> AAKRRPKEAEPEQVAPETPEDR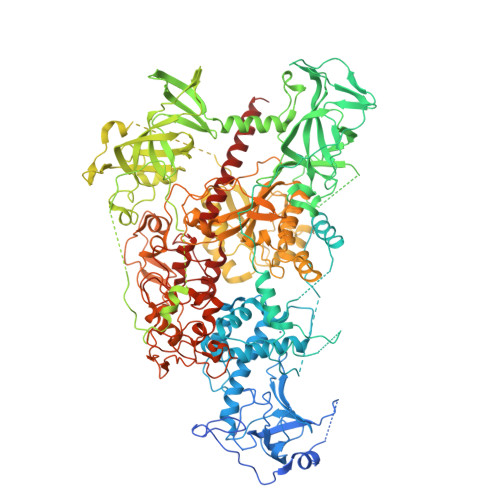DEDEREEKRRKTTRKKLESHTVPVQSRSERKAAQSKSVIPKINSPKCPECGQHLDDPNLKYQQHPEDAVDEPQMLTSEKLSIYDSTSTWFDTYEDSPMHRFTSFSVYCSRGHLCPVDTGLIEKNVELYFSGCAKAIHDENPSMEGGINGKNLGPINQWWLSGFDGGEKVLIGFSTAFAEYILMEPSKEYEPIFGLMQEKIYISKIVVEFLQNNPDAVYEDLINKIETTVPPSTINVNRFTEDSLLRHAQFVVSQVESYDEAKDDDETPIFLSPCMRALIHLAGVSLGQRRATRRVMGATKEKDKAPTKATTTKLVYQIFDTFFSEQIEKYDKEDKENAMKRRRCGVCEVCQQPECGKCKACKDMVKFGGTGRSKQACLKRRCPNLAVKEADDDEEADDDVSEMPSPKKLHQGKKKKQNKDRISWLGQPMKIEENRTYYQKVSIDEEMLEVGDCVSVIPDDSSKPLYLARVTALWEDKNGQMMFHAHWFCAGTDTVLGATSDPLELFLVGECENMQLSYIHSKVKVIYKAPSENWAMEGGTDPETTLPGAEDGKTYFFQLWYNQEYARFESPPKTQPTEDNKHKFCLSCIRLAELRQKEMPKVLEQIEEVDGRVYCSSITKNGVVYRLGDSVYLPPEAFTFNIKVASPVKRPKKDPVNETLYPEHYRKYSDYIKGSNLDAPEPYRIGRIKEIHCGKKKGKVNEADIKLRLYKFYRPENTHRSYNGSYHTDINMLYWSDEEAVVNFSDVQGRCTVEYGEDLLESIQDYSQGGPDRFYFLEAYNSKTKNFEDPPNHARSPGNKGKGKGKGKGKGKHQVSEPKEPEAAIKLPKLRTLDVFSGCGGLSEGFHQAGISETLWAIEMWDPAAQAFRLNNPGTTVFTEDCNVLLKLVMAGEVTNSLGQRLPQKGDVEMLCGGPPCQGFSGMNRFNSRTYSKFKNSLVVSFLSYCDYYRPRFFLLENVRNFVSYRRSMVLKLTLRCLVRMGYQCTFGVLQAGQYGVAQTRRRAIILAAAPGEKLPLFPEPLHVFAPRACQLSVVVDDKKFVSNITRLSSGPFRTITVRDTMSDLPEIQNGASNSEIPYNGEPLSWFQRQLRGSHYQPILRDHICKDMSPLVAARMRHIPLFPGSDWRDLPNIQVRLGDGVIAHKLQYTFHDVKNGYSSTGALRGVCSCAEGKACDPESRQFSTLIPWCLPHTGNRHNHWAGLYGRLEWDGFFSTTVTNPEPMGKQGRVLHPEQHRVVSVRECARSQGFPDSYRFFGNILDRHRQVGNAVPPPLAKAIGLEIKLCLLSSARESASAAVKAKEEAATKD> MEKIMPEEEYSEFKELILQKELHVVYALSHVCGQDRTLLASILLRIFLHEKLESLLLCTLNDREISMEDEATTLF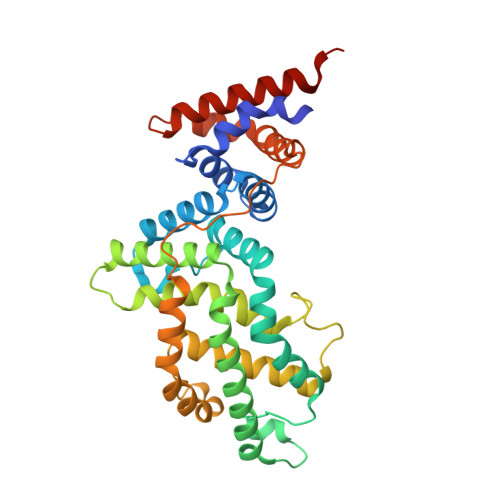RATTLASTLMEQYMKATATQFVHHALKDSILKIMESKQSCELSPSKLEKNEDVNTNLTHLLNILSELVEKIFMASEILPPTLRYIYGCLQKSVQHKWPTNTTMRTRVVSGFVFLRLICPAILNPRMFNIISDSPSPIAARTLILVAKSVQNLANLVEFGAKEPYMEGVNPFIKSNKHRMIMFLDELGNVPELPDTTEHSRTDLSRDLAALHEICVAHSDELRTLSNERGAQQHVLKKLLAITELLQQKQNQYTKTNDVR> MGHHHHHHSHMIRINEIKLPLDHEEGALLDAITKKLGIPAEKVISFNVFRRGYDARKKTNIHLIYTLDIIVEGDETALLAKFANDPHVRQTPDMEYKFVAKAPENLTERPIVIGFGPCGLFAGLVLAQMGFNPIIVERGKEVRERTKDTFGFWRKRTLNPESNVQFGEGGAGTFSDGKLYSQVKDPNFYGRKVITEFVEAGAPEEILYVSKPHIGTFKLVTMIEKMRATIIELGGEIRFSTRVDDLHMEDGQITGVTLSNGEEIKSRHVVLAVGHSARDTFEMLHERGVYMEAKPFSVGFRIEHKQSMIDEARFGPNAGHPILGAADYKLVHHCKNGRTVYSFCMCPGGTVVAATSEEGRVVTNGMSQYSRAERNANSAIVVGISPEVDYPGDPLAGIRFQRELESNAYKLGGENYDAPAQKIGDFLKGRDPSQLGDVEPSFTPGIKLTDLSKALPPFAVEAIREAIPAFDRKIKGFASEDGLLTGVETRTSSPVC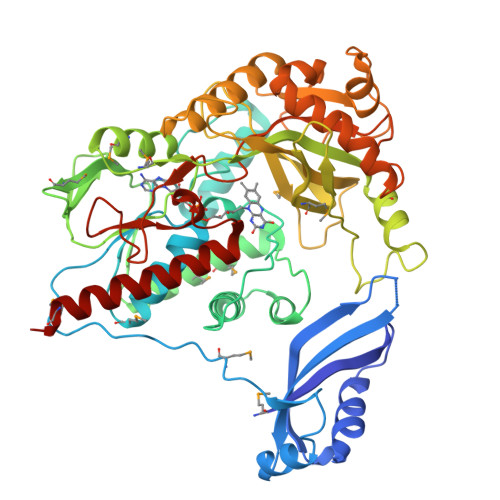IKRGKDFQSVNLKGFYPAGEGAGYAGGILSAGIDGIKVAEAVARDIVAAMENA>[2x]GSVTALSDVNNTDNYGAGQIQVLEGLEAVRKRPGMYIGSTSERGLHHLVWEIVDNSIDEALAGYANQIEVVIEKDNWIKVTDNGRGIPVDIQEKMGRPAVEVILTSSVVNA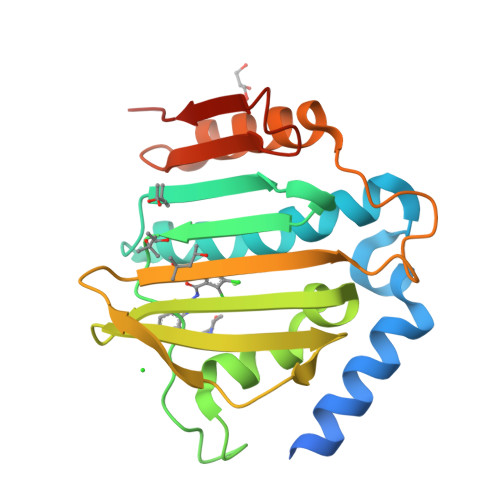LSQDLEVYVHRNETIYHQAYKKGVPQFDLKEVGTTDKTGTVIRFKADGEIFTETTVYNYETLQQRIRELAFLNKGIQITLRDERDEENVREDSYHYEGGIK> MTWPLPDRLSINSLSGTPAVDLSSFTDFLRRQAPELLPASISGGAPLAGGDAQLPHGTTIVALKYPGGVVMAGDRRSTQGNMISGRDVRKVYITDDYTATGIAGTAAVAVEFARLYAVELEHYEKLEGVPLTFAGKINRLAIMVRGNLA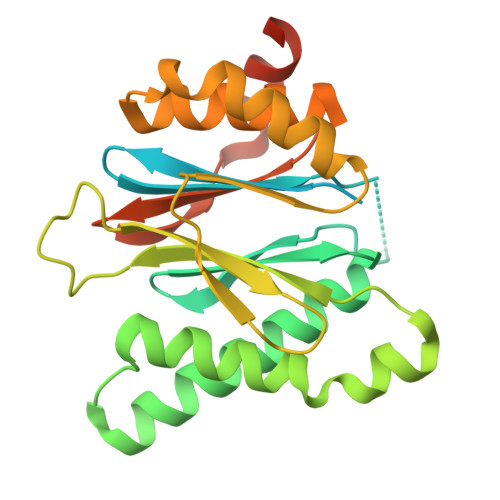AAMQGLLALPLLAGYDIHASDPQSAGRIVSFDAAGGWNIEEEGYQAVGSGSLFAKSSMKKLYSQVTDGDSGLRVAVEALYDAADDDSATGGPDLVRGIFPTAVIIDADGAVDVPESRIAELARAIIESRSGADTFGSDGGEK> MATLATHEDVTAFWARTPTAEEIVLINRRLAQAERMLLRAIPELLIKASSDPVFRAEVIDIEAEAVLRLVRNHEGYLSETDGNYTYMLQAQDPNRKLEILPEEWEVLGIVRSGLGILVP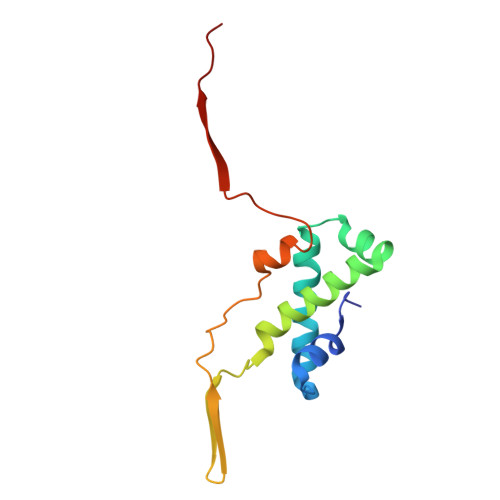TVVLPS>MTDIDVPQVADPEVAAMVRAEVEGRWPLGVSGLDEVVRYGLVPFGKMMGPWLLIRSALAVGGDIATALPAAVALECVQVGAMMHDDIIDCDAQRRSKPAAHTVFGEPTAIVGGDGLFFHGFAALSECREAGAPAERVAQAFTVLSRAGLRIGSAALREIRMSREICSVQDYLDMIADKSGALLWMACGVGGTLGGADEAALKALSQYSDQLGIAYQIRDDLMAYDGTRAGKPNISDVRNGRPTLPVLLAHERAPREQQLRIERLLADTAAPAAERYKAMADLVGAYDGAQ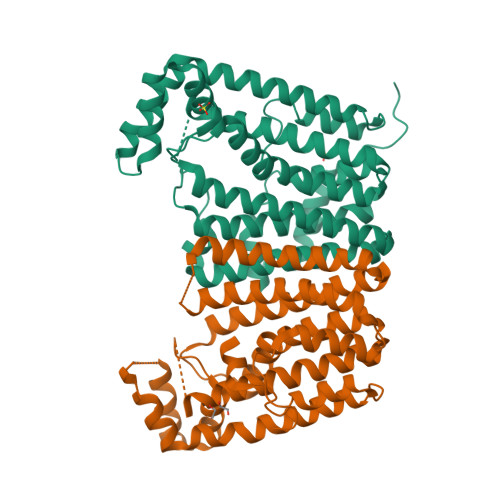AAREVSHRHVQLATRALQTLPPSPHRDALEDLTVPGRLVLEHHHHHH[4x]>[4x]MGSS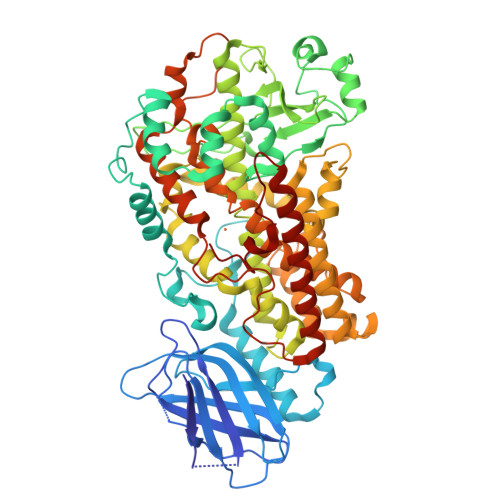HHHHHHSSGLVPRGSHMPSYTVTVATGSQEHAGTDDYIYLSLVGSAGCSEKHLLDKGSFERGAVDSYDVTVDEELGEIQLVRIEKRKYGSNDDWYLKYITLKTPHGDYIEFPCYRWITGDVEVVLRDGRAKLARDDQIHILKQHRRKELETRQKQYRWMEWNPGFPLSIDAKCHKDLPRDIQFDSEKGVDFVLNYSKAMENLFINRFMHMFQSSWNDFADFEKIFVKISNTISERVMNHWQEDLMFGYQFLNGANPVLIRRCTELPEKLPVTTEMVECSLERQLSLEQEVQQGNIFIVDFELLDGIDANKTDPCTLQFLAAPICLLYKNLANKIVPIAIQLNQIPGDENPIFLPSDAKYDWLLAKIWVRSSDFHVHQTITHLLRTHLVSEVFGIAMYRQLPAVHPIFKLLVAHVRFTIAINTKAREQLICECGLFDKANATGGGGHVQMVQRAMKDLTYASLCFPEAIKARGMESKEDIPYYFYRDDGLLVWEAIRTFTAEVVDIYYEGDQVVEEDPELQDFVNDVYVYGMRGRKSSGFPKSVKSREQLSEYLTVVIFTASAQHAAVNFGQYDWASWIPNAPPTMRAPPPTAKGVVTIEQIVDTLPDRGRSCWHLGAVWALSQFQENELFLGMYPEEHFIEKPVKEAMARFRKNLEAIVSVIAERNENLQLPYYYLSPDRIPNSVAI> TVSFNPYE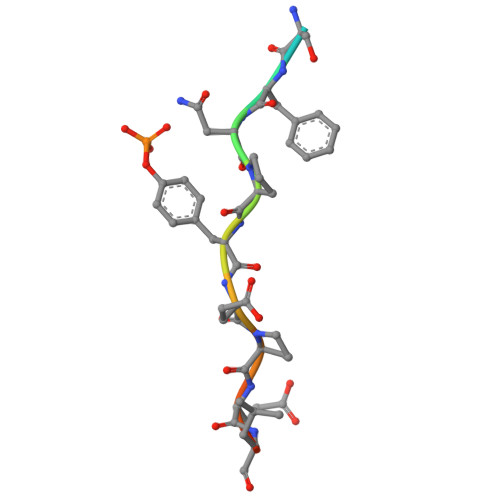PELAP>[2x]MRQVDAATHGGRAVIELREKILSGELPGGMRLFEVSTAELLDISRTPVREALSRLTEEGLLNRLPGGGFVVRRFGFADVVDAIEVRGVMEGTAARLAAERGVSKVALEEIDATVQQLDLCFG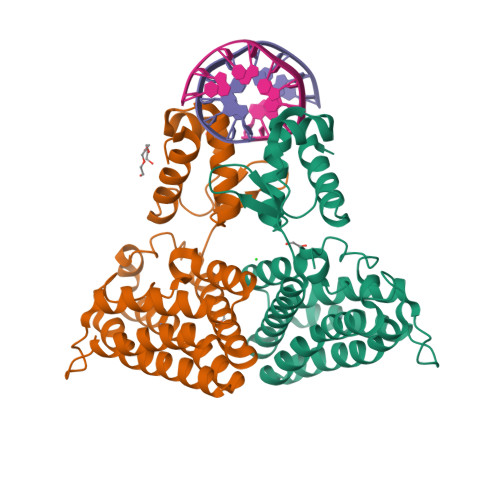DRVDDVDFDGYAALNRIFHHQLAALCGSEMIRREVERASSLPFASPSAFLPDKANIGAFRRSLRGAQEQHKAIVAAIVAREGARAEAVAREHSRTARTNLEYMIREAPELIAQVPGLALISDHHHHHH> MSGMPPRVRRRVEELLR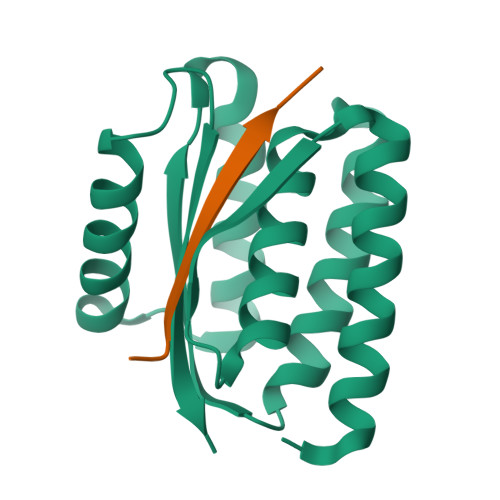RARELAEELGIRVEVLEVDPEYELELTAVITLAILAVLAPPERQDEVLELLRETLKTLSEVVESLAVSIWAPPEREEAARRVERLVEEAFNTTPETRERARKLRDEARRDAEPDEVVVAVHLVPKGSHHHHHH;> KPGFGVGRGLAPR> GASLKEIIDELGKQAKEQNKIASRILKIKGIKRIV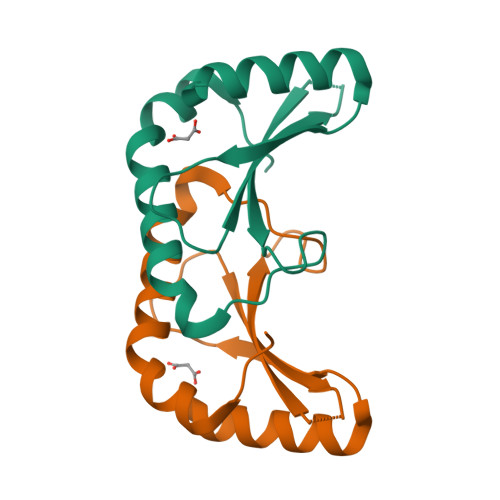VQLNAVPQDGKIRYSLTIHSQNNFRKQIGITPQDAEDLKLIAEFLEKYSDFLNEYVKFTPR>[2x]SNAMSSSLGDVLATLELERVGQWRFVGQQLPAPANHILGGHISAQALLAASRTAAGREPHSVHTYFLRPGDSRQPVDFEVVDLQEGRTFSARRVTARQDDKILMEAMSSFKVVNSAAAQVVYQPIMPEAPSPESLPWVA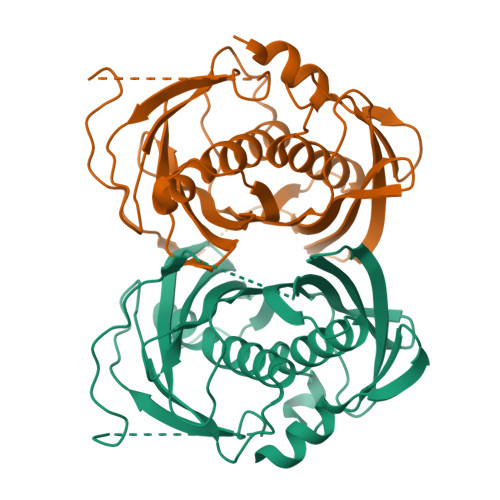PHLAEADEGSRGRWASLRWFERRTIETETVPPARVPMWWRPDGRVPDDPVLTASLVAYMSAVTLTEPAFAARGGVGASAQRDHSVWFHGRAVLSDWLFYDRSSPSSAGSLALASGTMFNRTGELVCTVKQEMYFPPQTA> MGSSHHHHHHEGEYIKLKV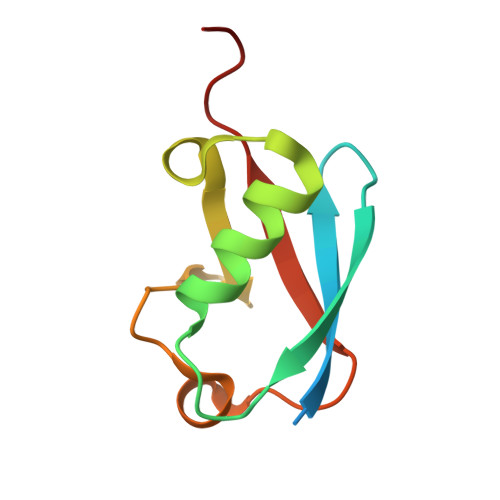IGQDSSEIHFKVKMTTHLKKLKESYCQRQGVPMNSLRFLFEGQRIADNHTPKELGMEEEDVIEVYQEQTGG> MSEWMKKGPLE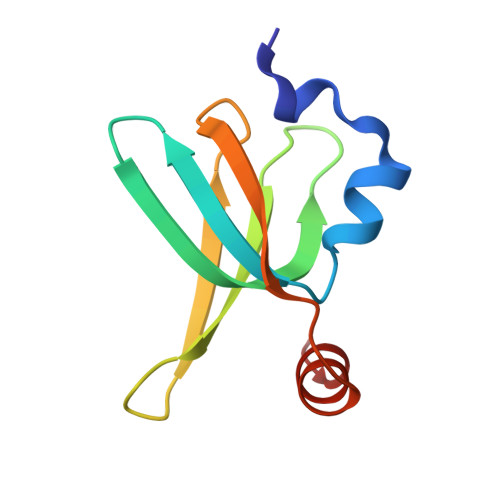WQDYIYKEVRVTASEKNEYKGWVLTTDPVSANIVLVNFLEDGSMSVTGIMGHAVQTVETMNEGDHRVREKLMHLF>MNLREKYGEWGLILGATEGVGKAFCEKIAAGGMNVVMVGRREEKLNVLAGEIRETYGVETKVV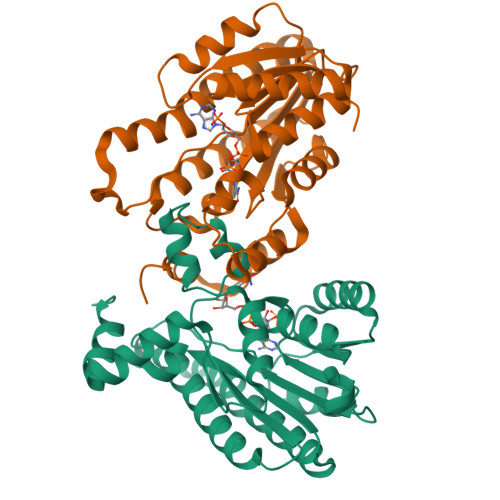RADFSQPGAAETVFAATEGLDMGFMSYVACLHSFGKIQDTPWEKHEAMINVNVVTFLKCFHHYMRIFAAQDRGAVINVSSMTGISSSPWNGQYGAGKAFILKMTEAVACECEGTGVDVEVITLGTTLTPSLLSNLPGGPQGEAVMKIALTPEECVDEAFEKLGKELSVIAGQRNKDSVHDWKANHTEDEYIRYMGSFYRD[2x]> AGQGDGSVIELGEQTVVATAQEETKQAPGVSIITAEDIAKRPPSNDLSQIIRTMPGVNLTGNSSSGQRGNNRQIDIRGMGPENTLILVDGKPVSSRNSVRYGWRGERDSRGDTNWVPADQVERIEVIRGPAAARYGNGAAGGVVNIITKQAGAETHGNLSVYSNFPQHKAE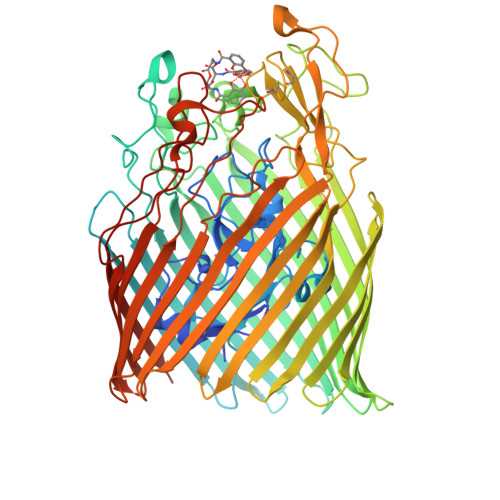GASERMSFGLNGPLTENLSYRVYGNIAKTDSDDWDINAGHESNRTGKQAGTLPAGREGVRNKDIDGLLSWRLTPEQTLEFEAGFSRQGNIYTGDTQNTNSNNYVKQMLGHETNRMYRETYSVTHRGEWDFGSSLAYLQYEKTRNSRINEGLAGGTEGIFDPNNAGFYTATLRDLTAHGEVNLPLHLGYEQTLTLGSEWTEQKLDDPSSNTQNTEEGGSIPGLAGKNRSSSSSARIFSLFAEDNIELMPGTMLTPGLRWDHHDIVGDNWSPSLNLSHALTERVTLKAGIARAYKAPNLYQLNPDYLLYSRGAGCYGQSTSCYLRGNDGLKAETSVNKELGIEYSHDGLVAGLTYFRNDYKNKIESGLSPVDHASGGKGDYANAAIYQWENVPKAVVEGLEGTLTLPLADGLKWSNNLTYMLQSKNKETGDVLSVTPRYTLNSMLDWQATDDLSLQATVTWYGKQKPKKYDYHGDRVTGSANDQLSPYAIAGLGGTYRLSKNLSLGAGVDNLFDKRLFRAGNAQGVVGIDGAGAATYNEPGRTFYTSLTASF>[5x]GPMAEKLNFEELNSMQRYSQFAVFRAIPGALGSDRAEIVAQA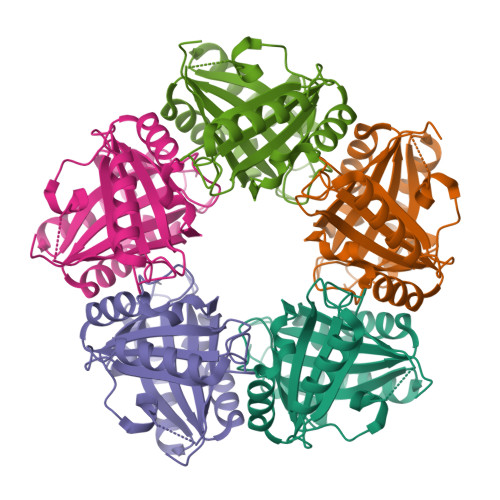QSFFDGLETAGKVEVRGIYDLAGCRAEADFMIWWIAEEFEEIQAAFARFRRETVLGQVSEVAWLGNSLHRPAEFNRSHLPSFIMGEIPGDWITVYPFVRSYDWYIMDPQKRRKILAEHGQAARDFPDVRANTVPAFALGDYEWMLAFEAPRLDRIVDLMHKMRYTEARLHVREETPFFTGRRVSEVSELVNVLPG> INIGNKTNENVISFFDSTDAETQN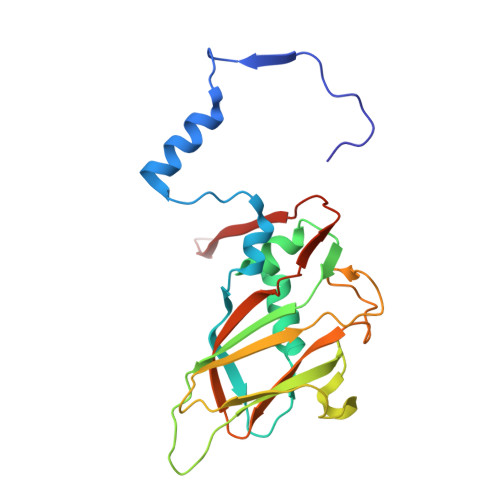HDVLMKGCGEFIVNLRTLLRTFRTITDNWILQANTKTPITDLTNTTDAQGRDYMSYLSYLYRFYRGGRRYKFFNTTPLKQSQTCYIRSFLMPRNYSADEINVDGPSHITYPVINPVHEVEVPFYSQYRKIPIASTSDKGYDSSLMYFSNTSTTQIVARAGNDDFTFGWMIGPPQLQGETRSVVP>MMSDASDMLAAALEQMDGIIAGSGSGSSPMHLQHIREQMAIALKRLKELEEQVRTIPVLQVKISVLQEEKRQLVSQLK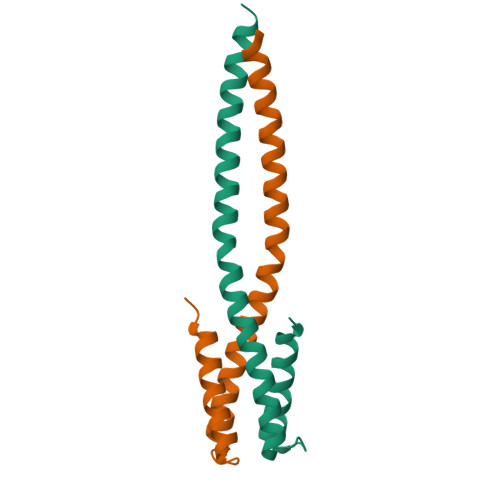NQRAASQINGLEHHHHHH[4x]> GSALSEIETRHSEIIK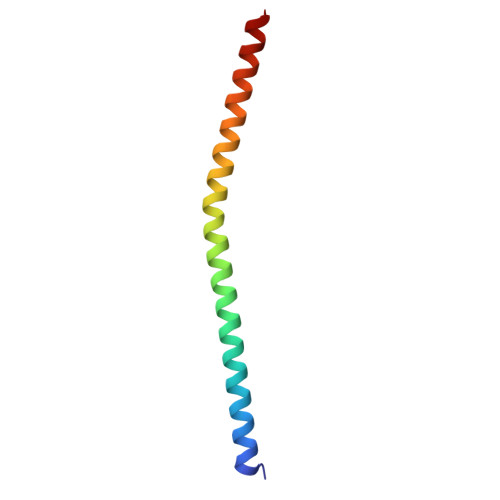LENSIRELHDMFMDMAMLVESQGEMIDRIEYNVEHAVDYVERAVSDTKKAVK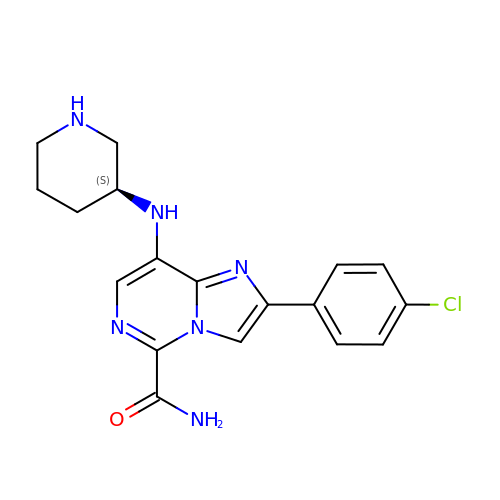2-(4-chlorophenyl)-8-[(3S)-piperidin-3-ylamino]imidazo[1,2-c]pyrimidine-5-carboxamide | C18 H19 Cl N6 O | VUQDZGWRLHHYTB-ZDUSSCGKSA-N> MGSQVSTQRSGSHENSNSATEGSTINYTTINYYKDSYAATAGKQSLKQDPDKFANPVKDIFTEMAAPLKSPSAEACGYSDRVAQLTIGNSTITTQEAANIIVGYGEWPSYCSDSDATAVDKPTRPDVSVNRFYTLDTKLWEKSSKGWYWKFPDVLTETGVFGQNAQFHYLYRSGFCIHVQCNASKFHQGALLVAVLPEYVIGTVAGGTGTEDSHPPYKQTQPGADGFELQHPYVLDAGIPISQLTVCPHQWINLRTNNCATIIVPYINALPFDSALNHCNFGLLVVPISPLDYDQGATPVIPITITLAPMCSEFAGLRQ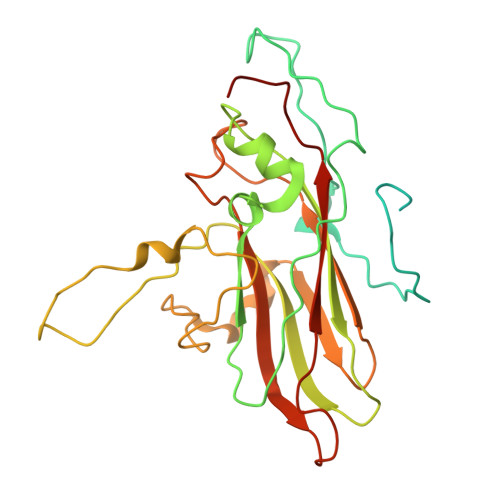AVTQ>MQAEKLGSEIKKI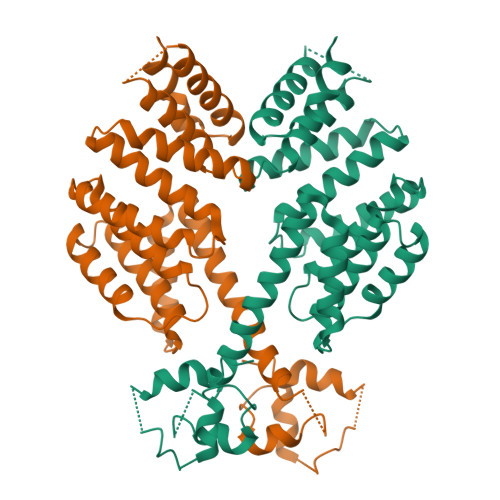RVLRGLTQKQLSENICHQSEVSRIESGAVYPSMDILQGIAAKLQIPIIHFYEVLIYSDIERKKQFKDQVIMLCKQKRYKEIYNKVWNELKKEEYHPEFQQFLQWQYYVAAYVLKKVDYEYCILELKKLLNQQLTGIDVYQNLYIENAIANIYAENGYLKKGIDLFEQILKQLEALHDNEEFDVKVRYNHAKALYLDSRYEESLYQVNKAIEISCRINSMALIGQLYYQRGECLRKLEYEEAEIEDAYKKASFFFDILEMHAYKEALVNKISRLEHHHHHH[4x]>[10x]MDNY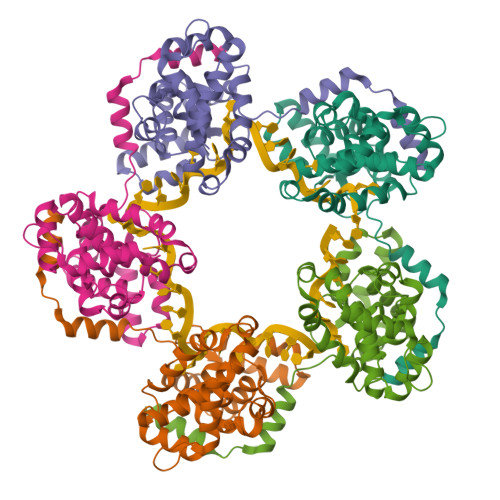QELAIQFAAQAVDRNEIEQWVREFAYQGFDARRVIELLKQYGGADWEKDAKKMIVLALTRGNKPRRMMMKMSKEGKATVEALINKYKLKEGNPSRDELTLSRVAAALAGRTCQALVVLSEWLPVTGTTMDGLSPAYPRHMMHPSFAGMVDPSLPGDYLRAILDAHSLYLLQFSRVINPNLRGRTKEEVAATFTQPMNAAVNSNFISHEKRREFLKAFGLVDSNGKPSAAVMAAAQAYKTAA> GAFGWEQDRGAPFSGRSPRILTRMTDAPRPTAGADAPARPPAAPLVAPNFITEIIERDLEAGKYPRVVTRFPPDPSGYAHLGHVFASLLDFNTARQYGGQFNLRMDDTNPELARQEYVDSIADDLKWLGLDWGEHFYYASDYFDRYYAYAEQLIRQGDAYVESVSPEELSRLRGNATTPGTPS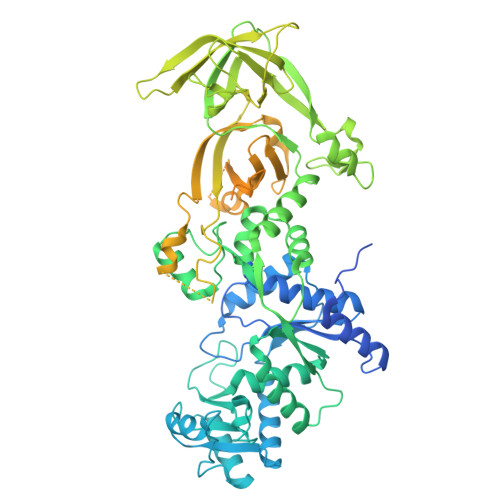PYRDRSVEENLDLLRRMKAGEFADGEHVLRAKIDLTAPNMKLRDPVLYRIVNKPHFRTSDEWHIYPAYDFEHPLQDAIEGVTHSMCSLEFVDNRAIYDWLMEKLNFDPRPHQYEFGRRGLEYTITSKRKLRELVQAGRVSGWDDPRMPTLRAQRRLGVTPEAVRAFAAQIGVSRTNRTVDIAVYENAVRDDLNHRAPRVMAVLDPVKVTLTNLDGEKTLSLPYWPHDVVRDSPDGLVGMPGGGRVAPEEAVRDVPLTRELYIERDDFSPAPPKGFKRLTPGGTVRLRGAGIIRADDFGTDEAGQVTHIRATLLGEDAKAAGVIHWVSAERALPAEFRLYDRLFRVPHPEGENADVEDDSAGPAEHEAEPGAGQETAPVSQGFMRYLTPDSLRVLRGYVEPSVAGDPADTRYQFERQGYFWRDPVELERVDSREDALVFGRIITLKDTWGKQGGGTQQKAEGKKRPSTKGRGPDEVRGEGSSSPAKAHAPKAQPLTPEQDAEFTRLLGLGASEGDARTIARDPALLAFVGGAAPGDTFAQVASWTVNELVAGLRAGEVKVRAADLAPLAEGVASGQLSARIAREALARAAASGDAPLTIIEREGLNAGLSAEALQQVVAQVIAANPDKAEAYRGGKTALLGFFTGQVMRATAGKADPQALAAALKDALA>[3x]MEGNTILKIVLICTILAGLFGQVVPVYAENTTYQTPTGIYYEVRGDTIYMINVTSGEETPIHLFGVNWFGFETPNHVVHGLWKRNWEDMLLQIKSLGFNAIRLPFCTESVKPGTQPIGIDYSKNPDLRGLDSLQIMEKIIKKAGDLGIFVLLDYHRIGCTHIEPLWYTEDFSEEDFINTWIEVAKRFGKYWNVIGADLKNEPHSVTSPPAAYTDGTGATWGMGNPATDWNLAAERIGKAILKVA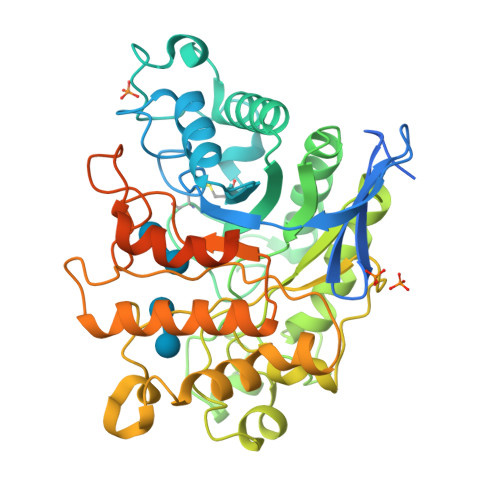PHWLIFVEGTQFTNPKTDSSYKWGYNAWWGGNLMAVKDYPVNLPKNKLVYSPHVYGPDVYNQPYFGPAKGFPDNLPDIWYHHFGYVKLELGYSVVIGEFGGKYGHGGDPRDVIWQNKLVDWMIENKFCDFFYWSWNPDSGDTGGILQDDWTTIWEDKYNNLKRLMDSCSKSSSSTQSVIRSTTPTKSNTSKKICGPAILIILAVFSLLLRRAPR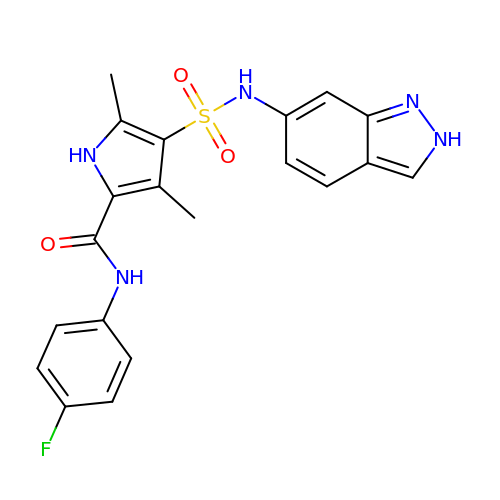~{N}-(4-fluorophenyl)-4-(2~{H}-indazol-6-ylsulfamoyl)-3,5-dimethyl-1~{H}-pyrrole-2-carboxamide | C20 H18 F N5 O3 S | LWWWROAXBQFQIU-UHFFFAOYSA-N> GG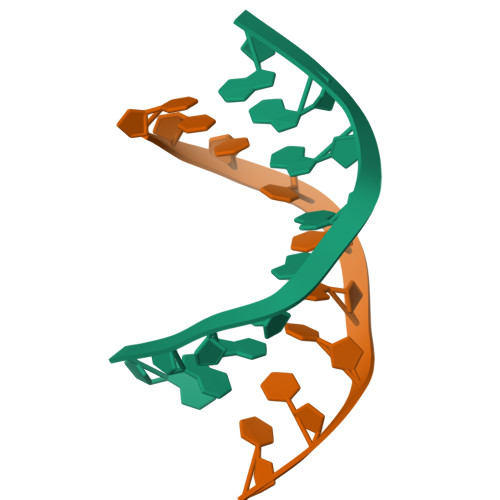ATGGGAG;> CTCCCATCC> MGSSHHHHHHSQDPMEIDELTALGGLLHDIGKPVQRAGLYSGDHSTQGARFLRDLAENTGRAEYELLSLFSEFHHKGHMKNDELMIRRIKELSPERFGLTMEDVLNALWIVYEADNLASGEREEGQPQASRPLYSVFNPGKAYPWAELDFEKELPVPGDVFSIRS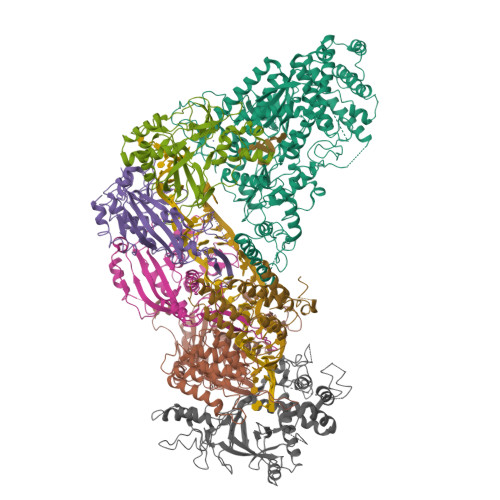QDYRELVKRLWEELSKAKLRSDRLLPVLEKYLTFVSSVTSEGNIISLYDHMRMTSAIALAMLRAGCTAEDVRSGRCRKEKRFLLIEGDFSGIQDFIYRVSGKGTLKYLRARSAYLELIGWDVVLEILSRLGLTRANVVFNAGGHFMIIAQNTPDAVKELEEIRAKAVEWLYREFESDLYLAIEWEPVSGREFGREGGKNLFAEARKRLKHKLTVRKLKRFGEIKGLFEHGHTERLAECPVCGRELPEGKLEPSASDPETKVCPTCNRLVSLGGNLPKLLGFGRTAKNDAGVLVEGPFSGFVPYLQGGRPVGEQILVKNTLNPGEIPESAQFVPYFVADYFKKDPKGGVATFEELSMASTGTRRLGVMKGDVDRLGEFFSSMDSPSKLATASRFMDYFFKGYIGAIIEGKFGYIIGDVPSLRDWPEEPDIVVVYAGGDAFFIVGAWDQIFELAFRVRRAFNAYTGGKLTLSVGLGYFDERTPIYRMADVVSERLDTAKDEGRNRVFVVGRSRPLDGKHKLSYEWNHYEELWRTYAPRIYAGNGRLKGKLESKKGLLWKLLEIRELYVRDPNDVRWAYLTAYLLGRHGLSDLFPELVGIDTKAVERKEPQPVYWVDGVLKIVLMAVRR;>[2x]SMAYHQKHGGYGRGGYGRQDRPQVDASRLFGESPDVVGIKKMLEGKGKQWEAIQPYFDNVVREAKNFLEWSPNKRLANAVTVAAYLTSQGLKTNQVRKILDMARTTELKVKRGEGDIKDDLVKMRYLLAYTVGKATGQSKYSLDAFHRILDPMLEVLMGSPKKENFEKFYDFLQAVVAYHKFFGGGD;>SMDRRFYGKIVIKGKIKAVTGLHIGSQRDISEIGGIDNPVIKDPHTGLPYIPGSSLKGRLRSLFEILVNSRLGEWREKYPSLANYSPGSCRPDNQENCGKFFNRKINRGWIHVCPDYETALACPVCRLFGASGKESNFPSRIIVRDAFLTKEWEEKWRAGEAITEAKIEVGIDRVTSQANPRTNERVVAGAEFEFEIIYNVENTTHWRDDIKNLLTAMALLEDSYLGGSGSRGYGKVKFIFDSFEFRPLDYYRTGKDEDIVSIDAREKSVSDILSGFDSLFSEVEGKLEAG[3x];> MPKFIAVKLIPKGPFRDIPRADTLFGAIGNAISAIHGQSAVEELVDAFVGGARISSAFPYSGDTYYLPKPLSVEPALEGILTGLDEEERYTTAKRLRKAKYLDLKNFELALRLRPFTIPEEIPYARVDVPRVVLDRVTQDSSIYFWEEIRFREKSGVYFLYSGPREVFDGYIAPAMRFLGDTGIGGKSTWGAGLFEVEFHEMKIDAPGSEYSVTLSNALPTKTPVLWRLLRKGGWSFGRRKPRMTFIAEGSIVKNDPGGMERLELGLSHEVYVYGLTFPLGVELPEGLE> MWIGVISLFPEMFKAITE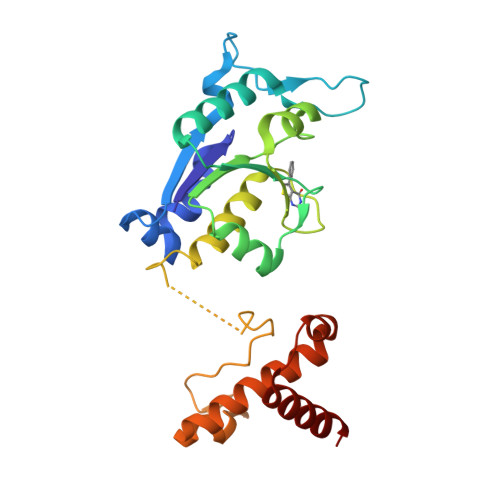FGVTGRAVKHNLLKVECWNPRDFTFDKHKTVDDRPYGGGPGMLMMVQPLRDAIHTAKAAAGEGAKVIYLSPQGRKLDQGGVTELAQNQKLILVCGRYEGIDERLIQTEIDEEWSIGDYVLTGGELPAMTLIDAVARFIPGVLGKQASAEEDSFADGLLDCPHYTRPEVLEGLTVPPVLMSGHHEEIRKWRLKQSLQRTWLRRPELLEGLALTDEQRKLLKEAQAEHNS>MSLAEGKWWRIMLVDTQLPALAASISALSQEGFDIIQCGNAIEAVPVAVKTHPHLIITEANMPKISGMDLFNSLKKNPQTASIPVIALSGRATAKEEAQLLDMGFIDFIAKPVNAIRLSARIKRVLKLLYEDLSAPPARE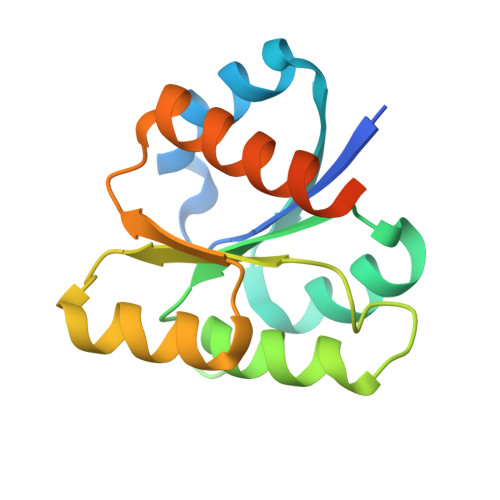GHHHHHH[2x]3-METHYL-2-OXOBUTANOIC ACID 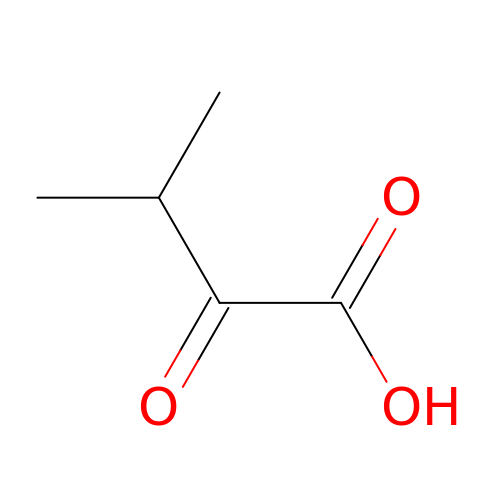| C5 H8 O3 | QHKABHOOEWYVLI-UHFFFAOYSA-N>[3x]MLEELKEANEYISSKIDKYKSPNLELIKEIEKDAEINNVPIISKEIREYLKFIIRTNKNIKNILEIGTAT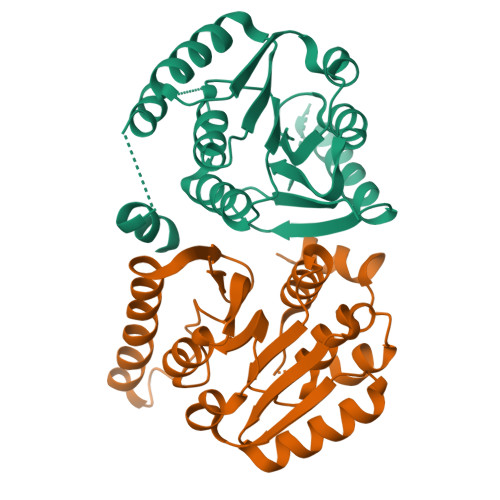GYSGIIMSEEIQGRNGTLTTIEIDEDRFKIAQSNFEKSNLKGIEQILGDATEEIEKLNKNFDFIFIDAAKGQYKKFFEDSYKLLNECGIVFVDNILFRGYLYKESPKRFKTIVKRLDEFVNYLYENFDFVLLPISDGVGIIHKPF>ATAVNGAPRDAALWSSHEQMLAQPLKDSDAEVYDIIKKESNRQRVGLELIASENFASRAVLEALGSCLNNKYSLGYPGQRYYGGTEHIDELETLCQKRALQAYGLDPQCWGVNVQPYSGSPANFAVYTALVEPHGRIMGLDLPDGGHLTHGFMTDKKKISATSIFFESMAYKVNPDTGYIDYDRLEENARLFHPKLIIAGTSCYSRNLDYGRLRKIADENGAYLMADMAHISGLVVAGVVPSPFEHCHVVTTTTHKTLRGCRAGMIFYRRGVRSVDPKTGKEILYNLESLINSAVFPGLQ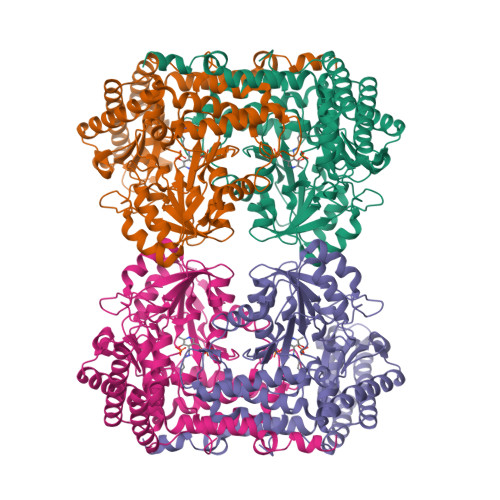GGPHNHAIAGVAVALKQAMTPEFKEYQRQVVANCRALSAALVELGYKIVTGGSDNHLILVDLRSKGTDGGRAEKVLEACSIACNKNTCPGDKSALRPSGLRLGTPALTSRGLLEKDFQKVAHFIHRGIELTVQIQDDTGPRATLKEFKEKLAGDEKHQRAVRALRQEVESFAALFPLPGLPGF[2x]>GSHMSSVTIGKCYIQNRENGGRAFYNLGRKDLGIFTGKMYD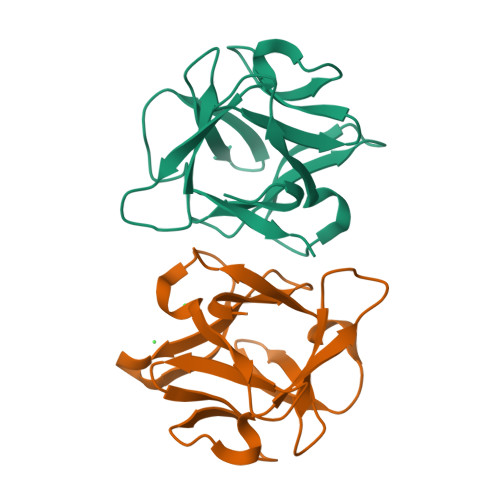DQIWSFQKSDTPGYYTIGRESKFLQYNGEQVIMSDIEQDTTLWSLEEVPEDKGFYRLLNKVHKAYLDYNGGDLVANKHQTESEKWILFKAY[2x]> MLAKRIIACLDVKDGRVVKGTNFENLRDSGDPVELGKFYSEIGIDELVFLDITASVEKRKTMLELVEKVAEQIDIPF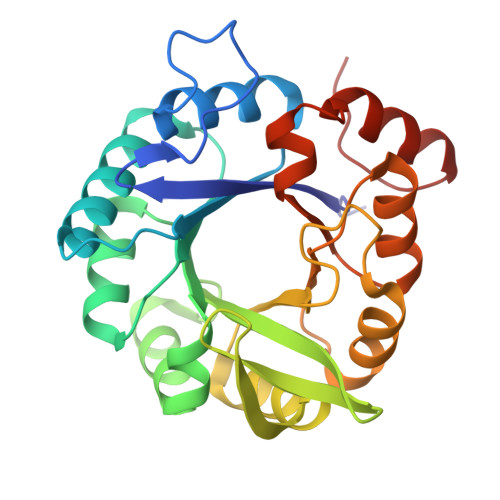TVGGGIHDFETASELILRGADKVSINTAAVENPSLITQIAQTFGSQAVVVAIDAKRVDGEFMVFTYSGKKNTGILLRDWVVEVEKRGAGEILLTSIDRDGTKSGYDTEMIRFVRPLTTLPIIASGGAGKMEHFLEAFLAGADAALAASVFHFREIDVRELKEYLKKHGVNVRLEGL MJ0927 is a member of the Nif3 family and is highly conserved among bacteria and humans. The crystal structure of MJ0927 determined at 2.47 Å revealed that MJ0927 folds into two interlinked α/β domains. Six protomers of MJ0927 are found to form a novel hollow cage-like hexamer, in contrast to the toroid-shaped hexamers formed by other members of the Nif3 family. Additionally, we found that MJ0927 is a DNA-binding protein exhibiting the ability to bind to both single-stranded DNA (ssDNA) and double-stranded DNA (dsDNA).

Two crystal forms of MJ0927 were obtained, one in the P21 and the other in the C2221 space groups. The Se-Met labeled P21 crystal structure was solved at 2.8 Å resolution by using the multiwavelength anomalous diffraction (MAD) method. The P21 crystal form contains six molecules in each asymmetric unit, forming a hexameric spheroid with a 32-symmetry. The six independent molecules in the asymmetric unit superpose well with pairwise root-mean-square deviations (rmsd) ranging from 0.222 to 0.310 Å. The MJ0927 hexamer can be described as two stacked trimers, consisting of monomers A-B-C and D-E-F, which are related by a two-fold symmetry. Contacts between molecules A and D, B and E, or C and F occur through the interdimer interactions. The surface area of each subunit buried in the interdimer interface is 1207 Å2, which constitutes ~10% of each subunit surface area. The hexamer is stabilized by a combination of interdimer and intratrimer interactions. These results are consistent with the previous gel filtration experiment showing that MJ0927 exists as a hexamer in solution. No significant structural differences of the individual molecules were observed between the P21 and C2221 crystal forms.

>[6x]MKAKEIIEFIETFAPKDLAIEGDNIGLQVGDNLDKEIKKLGIALDPSLSVIKKAEKEGVDFLFTHHPLLKDPIRNFTGVIYKKLKILMENDIILYSAHTNLDICKNGLNDALAELYNLENPKPLYDNGLGRVGIFKGSFEEFLEITKKYIHKNPIVVKSKEVDDNFKLAVLSGYGLSQSSIKYVAEKADVYLSGDLTHHSKILAEELGLVVVDATHYSTEVFGLKKFKEFLSSNLDLEIISLDFLEHHHHHH> NPASPPEEGSPDPDSTGALVEEEDPFFKVPVNKLAAAVSNFGYDLYRVRSSMSPTTNVLLSPLSVATALSALSLGADERTESIIHRALYYDLISSPDIHGTYKELLDTVTAPQKNLKSASRIVFEKKLRIKSSFVAPLEKSYGTRPRVLTGNPRLDLQEINNWVQAQMKGKLARSTKEIPDEISILLLGVAHFKGQWVTKFDSRKTSLEDFYLDEERTVRVPMMSDPKAVLRYGLDSDL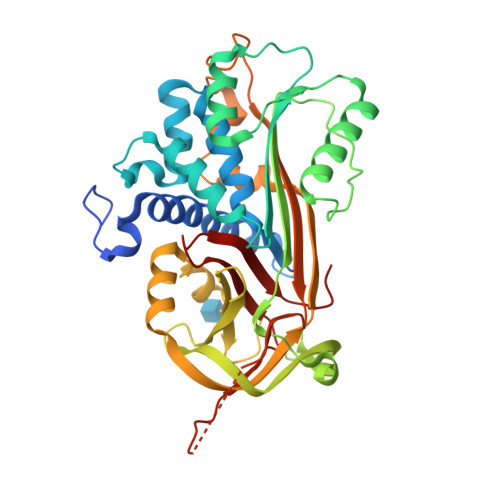SCKIAQLPLTGSMSIIFFLPLKVTQNLTLIEESLTSEFIHDIDRELKTVQAVLTVPKLKLSYEGEVTKSLQEMKLQSLFDSPDFSKITGKPIKLTQVEHRAGFEWNEDGAGTTPSPGLQPAHLTFPLDYHLNQPFIFVLRDTDTGALLFIGKILDPRGP>NSGMLEEDLIQYYQFLAEKGDVQAQVGLGQLHLHGGRGVEQNHQRAFDYFNLAANAGNSHAMAFLGKMYSEGSDIVPQSNETALHYFKKAADMGNPVGQSGLGMAYLYGRGVQVNYDLALKYFQKAAEQGWVDGQLQLGSMYYNGIGVKRDYKQALKYFNLASQGGHILAFYNLAQMHASGTGVMR[4x]

SEL1L, the mammalian homolog of Hrd3p, associates with HRD1, mediates HRD1 interactions with the ER luminal lectin OS9, and recognizes substrates to be degraded. SEL1L is required for ER homeostasis, which is essential for protein translation, pancreatic function, and cellular and organismal survival. Previous biochemical studies reveal that SEL1L is a type I transmembrane protein and has a large luminal domain comprising sets of repeated Sel1-like (SLR) motifs. The SLR motif is a structural motif that closely resembles the tetratricopeptide-repeat (TPR) motif, which is a protein-protein interaction module19.

We found that the central domain of SEL1L, comprising SLR motifs 5 through 9 (SEL1Lcent), forms a tight dimer with two-fold symmetry due to domain swapping of the SLR motif 9. Crystals of SEL1Lcent grew in space group P21 with four copies of SEL1Lcent (a total of 82 kDa) in the asymmetric unit. The assignment of residues during model building was aided by the selenium atom positions, and the structure was refined with native data to 2.6 Å resolution with Rwork/Rfree values of 20.7/27.7%. The two SEL1Lcent molecules dimerize in a head-to-tail manner through a two-fold symmetry interface resulting in a cosmos-like shaped structure. Each protomer is composed of ten α-helices, which form the five SLRs, resulting in an elongated curved structure, confirming the primary structure prediction. However, the last helix, 9B, at the C-terminus adopts a different conformation, lying parallel to the long axis of helix 9A instead of forming an antiparallel SLR. Helix 9B from one protomer inserts into the empty space surrounded by the concave region in the other monomer, forming a domain-swapped conformation. In this interface, Leu 516 and Tyr 519 on helix 9B are located in the center, making hydrophobic interactions with Trp 478 on helix 8B, Val 444 on helix 7B, Phe 411 on helix 6B, and Leu 380 on helix 5B from the SEL1Lcent counterpart (Interface 1 detail). For this structural geometry, two adjacent residues, Gly 512 and Gly 513, in SEL1L confer flexibility at this position by adopting main-chain dihedral angles that are disallowed for non-glycine residues. Notably, a single-residue mutation (L521A in interface 3) abolished the dimerization of SEL1Lcent.>SHMLIRKLFKFENAHVVRNCTSDRCKRSIHGHSYKVELLLKASKLDHGQMVYDFGLLKGVIKDLFDSFDHAICFWEKDDPQYIDACKTFSARWISLPVSPSAEQFSRIFFYLAQQ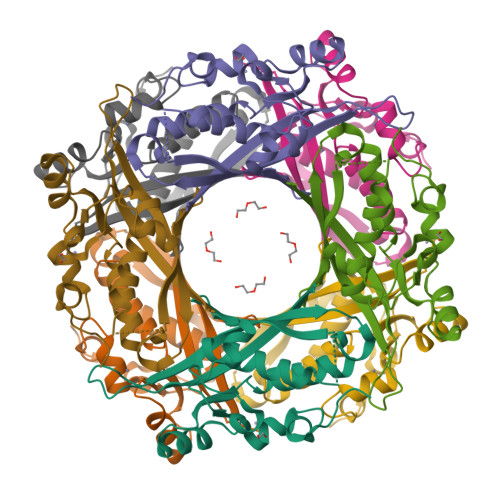VLQSTVTQNGEGDVEVYSVIVHETDTGYAQSFLEDIQNEQMGLLNLEGIIFSEQVQSEWADPNMYENLKQGIKFHNPHVNLQVEV[2x]> GPLGSETYDFLFKFLVIGNAGTGKSCLLHQFIEKKFKDDSNHTIGVEFGSKIINVGGKYVKLQIWDTAGQERFRSVTRSYYRGAAGALLVYD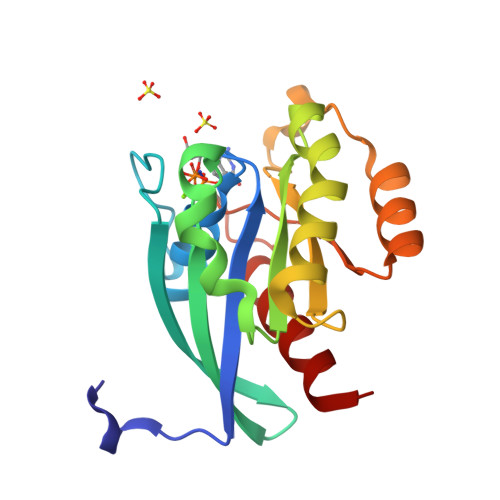ITSRETYNALTNWLTDARMLASQNIVIILCGNKKDLDADREVTFLEASRFAQENELMFLETSALTGEDVEEAFVQCARKILNK>[4x]MAEIKHYQ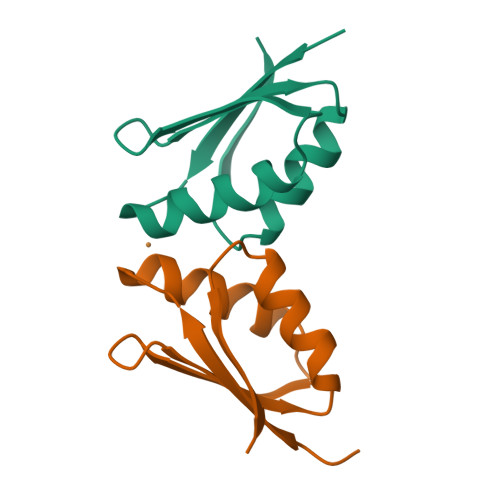FNVVMTCSGCSGAVNKVLTKLEPDVSKIDISLEKQLVDVYTTLPYDFILEKIKKTGKEVRSGKQL> GGATTA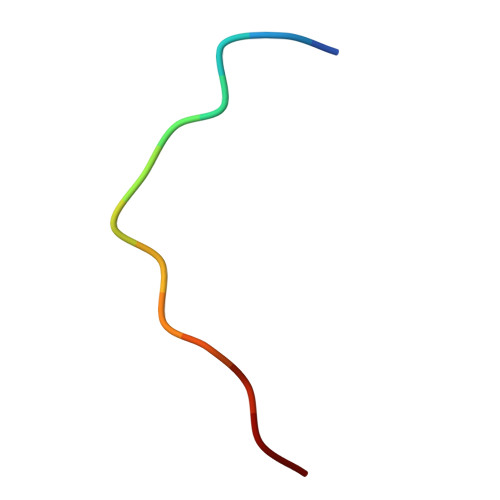TTTTSTS>[6x]MTETLPPVTESAVALQAEVTQRELFEFVLNDPLLASSLYINIALAGLSILLFVFMTRGLDDPRAKLIAVSTILVPVVSIASYTGLASGLTISVLEMPAGHFAEGSSVMLGGEEVDGVVTMWGRYLTWALSTPMILLALGLLAGSNATKLFTAITFDIAMCVT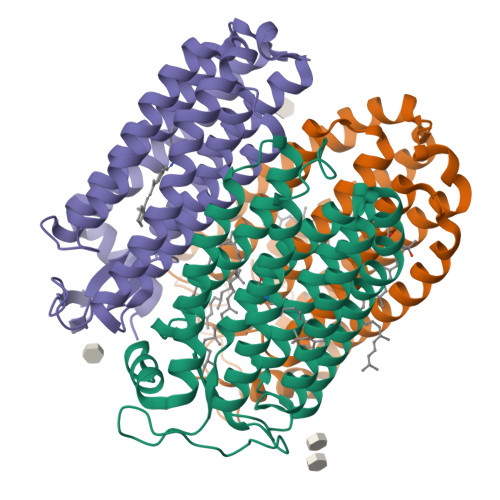GLAAALTTSSHLMRWFWYAISCACFIVVLYILLVEWAQDAKAAGTADIFSTLKLLTVVMWLGYPIVWALGVEGVAVLPVGYTSWAYSALDIVAKYIFAFLLLNYLTSNEGVVSGSILDVPSASGAPADD> MTKLKAPAVLAYSRKINPTNALMFAVNWSDRDNT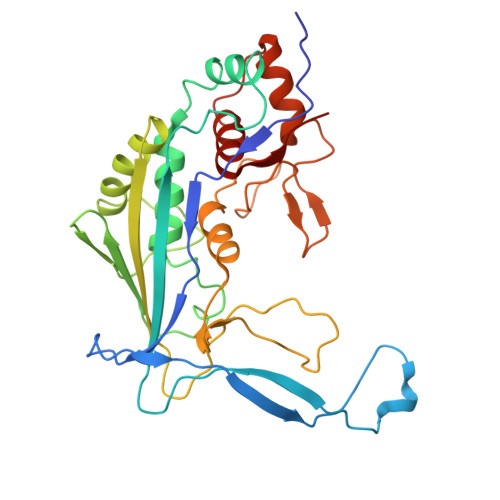TAVMVGTKTVAGTQSVRGNPNDADKGNIQTVNFANLPHNKNTLLVKYNVKFVGDVFKAELGGGEYSNTLQTALENTDFGTLAYRYVYNIAAGRTLWRNRVGAESIETVITVNDQTFTFSDLLVNEFDEDVDVAEIADMVAGVLSGEGFVTLKVEHYMLLGEGSEVFPSQEFVENSKLSKQLFDLNGQAAMHDQKIGNAIRTIDTWYEDATTPIAVEPYGSVVRNGVAYRAGNKTDLFTLMDGAVNGKSLTEEDQMFVTANLIRGGVFGGGKD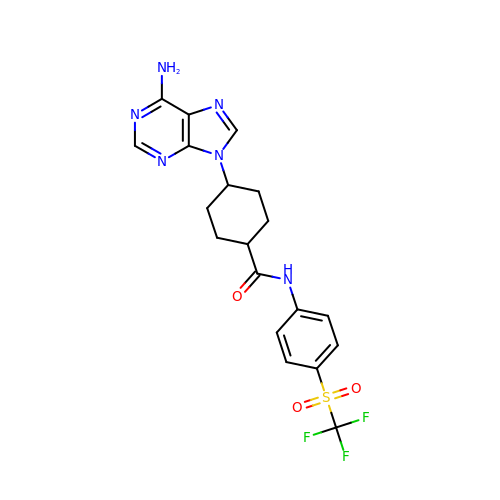4-(6-aminopurin-9-yl)-~{N}-[4-(trifluoromethylsulfonyl)phenyl]cyclohexane-1-carboxamide | C19 H19 F3 N6 O3 S | QWZUCMUBFGMZFO-BJHJDKERSA-N>MAHHHHHHMPHALITLSADITEEIKKEIAHESMKILSEVIGKPISYCATQVVTSVGGFGGKIVKSAFIDIKSISGLKGKQEGLSDRYCKLLEQKAGIEGGNIYLNFTEMTGNNWGYDHST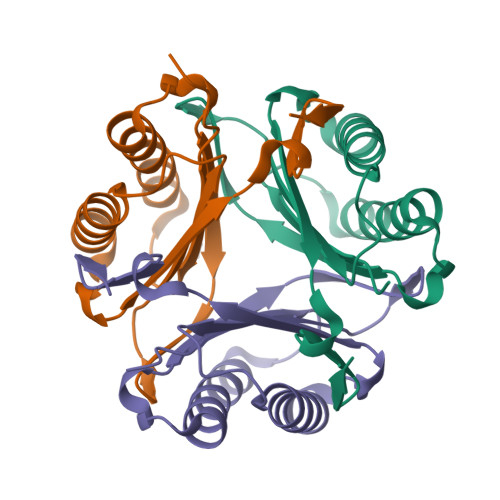F[3x]>MKKTQTWILTCIYLQLLLFNPLVKTEGICRNRVTNNVKDVTKLVANLPKDYMITLKYVPGMDVLPSHCWISEMVVQLSDSLTDLLDKFSNISEGLSNYSIIDKLVNIVDDLVECVKENSSKDLKKSFKSPEPRLFTPEEFFRIFN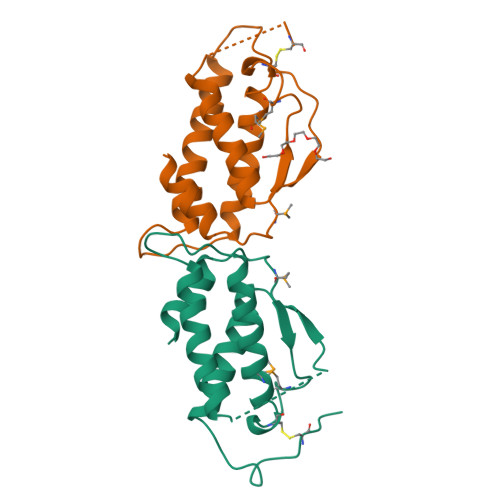RSIDAFKDFVVASETSDCVVSSTLSPEKDSRVSVTKPFMLPPVAASSLRNDSSSSNRKAKNPPGDSSLHWAAMALPALFSLIIGFAFGALYWKKRQPSLTRAVENIQINEEDNEISMLQEKEREFQEV[4x]N-(1H-benzimidazol-2-yl)-N'-(3,5-dichlorobenzyl)propane-1,3-diamine 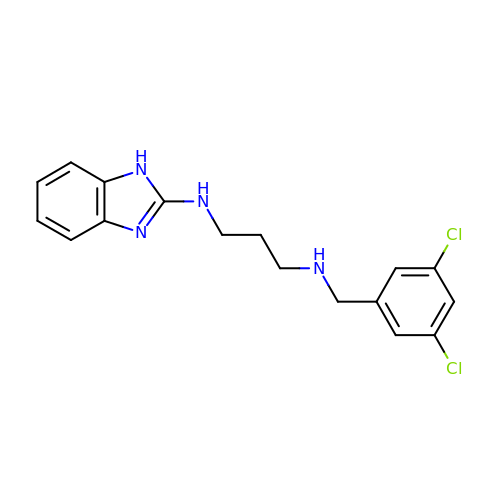| C17 H18 Cl2 N4 | ZITVWTWUGXKZFV-UHFFFAOYSA-N> 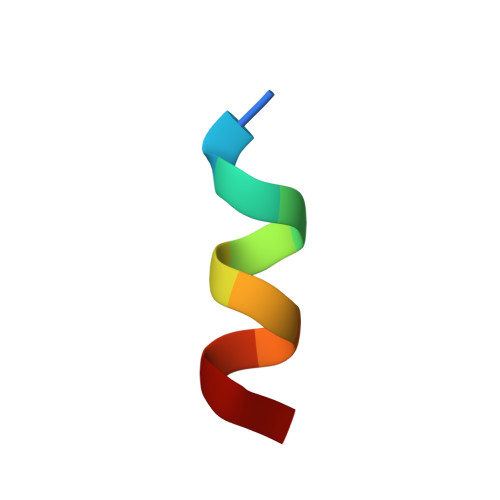KKALKKLAKLL> HMLEAKFEEASLFKRIIDGFKDCVQLVNFQCKEDGIIAQAVDDSRVLLVSLEIGVEAFQEYRCDHPVTLGMDLTSLSKILRCGNNTDTLTLIADNTPDS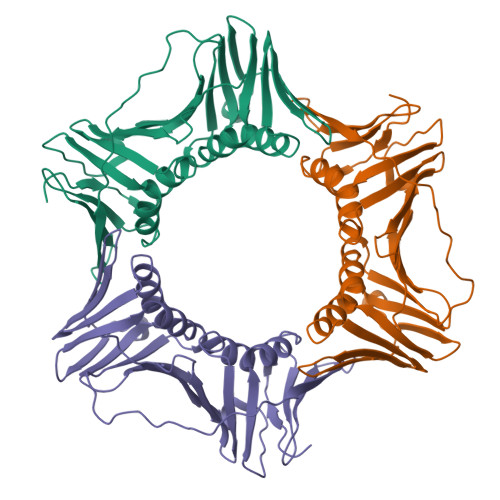IILLFEDTKKDRIAEYSLKLMDIDADFLKIEELQYDSTLSLPSSEFSKIVRDLSQLSDSINIMITKETIKFVADGDIGSGSAIIKPFVDMEHPETSIKLEMDQPVDLTFGAKYLLDIIKGSSLSDRVGIRLSSEAPALFQFDLKSGFLQFFLAPKFNDEE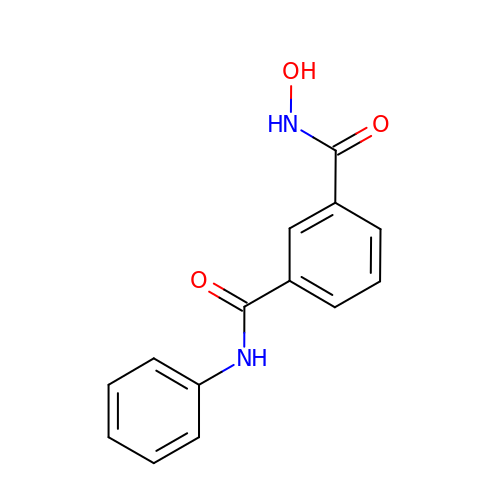~{N}1-oxidanyl-~{N}3-phenyl-benzene-1,3-dicarboxamide | C14 H12 N2 O3 | NXHPVXNYPQJIOB-UHFFFAOYSA-N> MIMEIPAIKALSRYAQWVIWKKERDTKIPYNPNNGKKASSTDPLAWGDIDEAQAGLVRYGANGLGFVLTKSDPFVFIDLDHVLDENKRVKCEWARQLLKEIKSYTEISPSGDGLHVVVSGKLPDYIKHKTKFDDGSALEVYESGRYMTITGEVFDGRDDIKELDLSILGEFAEHKIETKNAPVQIESATTLDDEAIIDLMKRKGQW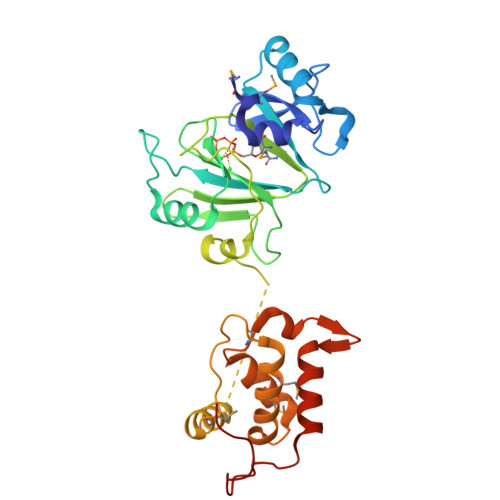PDAPADGDDWSSLDMSFANRLAFWCGKDIERMDRIFRQSPLMRQKWDRPTAGSTYGRITLKKACDFVDSVYDPALRNESDCPF>MNSSKETKSEPSDSKKLMDQPYSKTDFLMGTVVTLKIYDKGKEDVLDKGFDRIKDLAAKITTSDSEKTSEVDKINEQAGKKPVKVSEDVYYLIQEGLKYSENSGGSFDITIGPLTSLWHIGFSDARKPSQAEIDAVLPLINYKDVKMNDKDQTVYLEKEGMELDLGAIAKGFITDETLKVFKENKVTTSIIDLGGNIYVQGNNPNGNKWNVGIQDPFSPRGSVIGKLPESNMSIVTSGIYERYLEVDGKTYHHILDPKTGYPFDNDIAGVSIVSKKSIDGDGLSTATFSKGIKGGMDYIEQFEGVDAIFISKEKKVYETSGLKGQFELTDKDFQMDTLKK[2x]

A Mg2+‐dependent protein flavin mononucleotide (FMN) transferase (FmnB; UniProt: LMRG_02181) in EET is responsible for the transfer of electrons from intracellular to extracellular by hydrolyzing cofactor flavin adenine dinucleotide (FAD) and transferring FMN. FmnB is a flavin transferase belonging to ApbE family; it hydrolyzes flavin adenine dinucleotide (FAD) and converts flavin mononucleotide (FMN) to pheromone lipoprotein (PplA; UniProt: LMRG_02182), and divalent cations are required this process. Here, we report a series of crystal structures of apo‐FmnB and FmnB complexed with substrate FAD, three inhibitors AMP, ADP, and ATP, revealing the unusual catalytic triad center (Asp301‐Ser257‐His273) of FmnB. Notably, the structures of FmnB in complex with distinct inhibitors, together with biochemical assays, revealed that all three inhibitors indeed inhibited the activity of FmnB by occupying the binding site of the FAD substrate.

For FmnB‐ADP, the phosphate groups of ADP form salt bridges with Lys190 and His273 and a water‐mediated hydrogen bond with Thr305. Similarly, the Mg2+ ions near the ADP coordinate Asp301, Ala187, Asn216, and the phosphate groups as well as water molecules. Furthermore, while FmnB‐ADP is similar to FmnB‐AMP, the binding pocket for ADP is smaller, and there are no significant conformational changes in Met49 and Phe142. In particular, Arg262 is more distant (4.3 Å) from the β‐phosphate group of ADP, possibly due to spatial repulsion between Arg262 and the phosphate group. Remarkably, the structures revealed that the key residue Arg262 of FmnB was profoundly affected by ADP but not AMP or ATP. Moreover, considering the effect of Arg262, only the presence of ADP causes Arg262 to move away from the center of the cavity. Curiously, ADP exhibited a stronger inhibition ability than AMP and ATP. In summary, these charge repulsion and space constraints result in the strongest inhibition of FmnB enzyme activity by ADP compared with that by AMP and ATP.5-ALPHA-ANDROSTANE-3-BETA,17-ALPHA-DIOL | C19 H32 O2 | 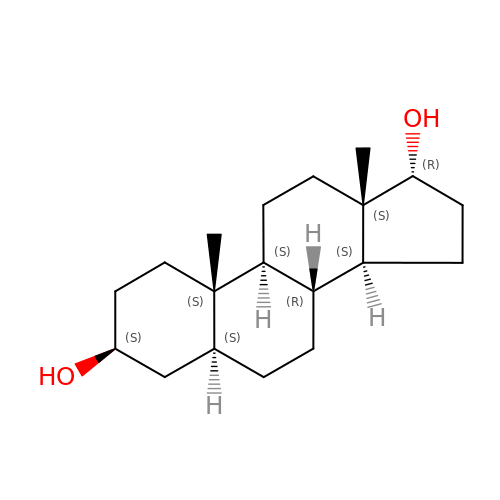CBMYJHIOYJEBSB-MFXFBURESA-N>[2x]LTSELAAQVRDAFDDDRDAETFLLRLERYGEDLWESLRAVYGDQVRALPGRLLEVMLHAYHARPAELRRLDEARLLRPDWLQRPEMVGYVAYTDRFAGTLKGVEERLDYLEGLGVKYLHLMPLLRPREGENDGGYAVQDYRAVRPDLGTMDDLSALARALRGRGISLVLDLVLNHVAREHAWAQKARAGDPKYRAYFHLFPDRRGPDAFEATLPEIFPDFAPGNFSWDEEIGEGEGGWVWTTFNSYQWDLNWANPDVFLEFVDIILYLANRGVEVFRLDAIAFIWKRLGTDCQNQPEVHHLTRALRAAARIVAPAVAFKAEAIVAPADLIHYLGTRAHHGKVSDMAYHNSLMVQLWSSLASRNTRLFEEALRAFPPKPTSTTWGLYVRCHDDIGWAISDEDAARAGLNGAAHRHFLSDFYSGQFPGSFARGLVFQYNPVNGDRRISGSAASLAGLEAALETGD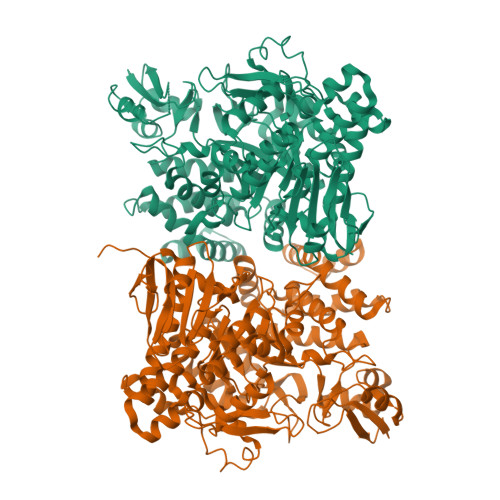PGRIEDAVRRLLLLHTVILGFGGVPLLYMGDELALLNDYAFEDVPEHAPDNRWVHRPQMDWALAERVRQEPSSPAGRVNTGLRHLLRVRRDTPQLHASIESQVLPSPDSRALLLRRDHPLGGMVQVYNFSEETVMLPSHVLRDVLGDHVQDRLSGSAFRLDRPTVRLEGYRALWLTAGEAPA The MSP signaling involves four consecutive phosphorylation events at: (i) the kinase domain of the sensory histidine kinase, (ii) the receiver domain of the latter protein, (iii) the histidine-containing phosphotransfer protein, and (iv) the response regulator. The second element in the MSP system, AHP, receives a signal (phosphate) from the receiver (REC) domain of HK and translocates into the nucleus to phosphorylate the REC domain of the RR. ARR1, a type-B ARR, contains the GARP domain for DNA binding, in addition to the canonical receiver domain that mediates AHP1 interaction. To bring new insights at the molecular level, we investigated the structural and biophysical characteristics of the AHP1/ARR1 complex.

The asymmetric unit (ASU) includes two complexes, each consisting of one AHP1 molecule and one ARR1-RG. While the electron density map clearly defines the entire AHP1 proteins, the region spanning 77 residues (from 159 to 235) in ARR1-RG is not visible, indicating the flexibility of the fragment that links the REC domain and the GARP motif. ARR1-RG contains the REC domain (residues 38-158) and the GARP motif (residues 236-296). Notably, the α3 helix is slightly bent compared with that in the published GARP structure of ARR10 (Hosoda et al., 2002). Despite being separated by 77 residues (159-235) in the ARR1 sequence, the REC domain and GARP motif interact with one another through a vast interface of 1044 Å2 [calculated by PDBePISA], as shown in Figure 2B . The Tyr291 residue from the GARP motif reaches deep into a hydrophobic pocket of the REC domain (inset). In other words, because part of the GARP interface that binds DNA is also involved in the GARP-REC interdomain interaction, GARP must be set free for it to bind DNA. AHP1 is composed of six helices with various lengths (from 3 to 10 turns), in which helices α3-α6 form a four-helix bundle. The phosphorylatable His79 (Ruszkowski et al., 2013) in helix α4 is exposed towards the ARR1 recognition site, which is highly conserved among type-B ARRs. In the case of ARR1, it is composed of the catalytic Asp89 at the C-terminus of the β3 strand, the double Asp motif (43-44) in the loop between β1 and α1, Ser116 at the C-terminus of β4, and Lys138 in the loop between β5 and α5. ARR1-RG binds AHP1 with a 1:1 stoichiometry through a relatively small interface of 875 Å2.

>[2x]SNAMDLVQKQKSLQDYTKSLFLEGILDSQFLQLQQLQDESNPDFVSQVVTLFFQDSDRILNDLSLSLDQQVVDFKKVDPHVHQLKGSSSSIGAQRVKNACVVFRSFCEQQNVEACHRCLQQVKQEYYLVKNRLETLFKLEQQIVASGGMIPAVELGF;>MHHHHHHENLYFQSNARVLVVDDDPTCLMILERMLRTCLYEVTKCNRAEMALSLLRKNKHGFDIVISDVHMPDMDGFKLLEHVGLEMDLPVIMMSADDSKSVVLKGVTHGAVDYLIKPVRMEALKNIWQHVVRKRRSEWSVPEHSGSIEETGERQQQQHRGGGGGAAVSGGEDAVDDNSSSVNEGNNWRSSSRKRKDEEGEEQGDDKDEDASNLKKPRVVWSVELHQQFVAAVNQLGVEKAVPKKILELMNVPGLTRENVASHLQKYRIYLRRLG[2x]>[6x]MPEQAVTLEALYAAIEQVLRERLPEAQLIGFWPGVPENTPAVSLEIAELLPERDPGTGESALLCRLQARIMVPPGADRQAVSIACGIVRTLREQTWNLSLQPARFVRSAVDGSREELKSLRVWLVEWTQSLRLGDPEWAWEDQPPGSLMLGFDPQTGPGHEPDYFAPEALA;>[18x]MSFFHGVTVTNVDIGARTIALPASSVIGLCDVFTPGAQASAKPNVPVLLTSKKDAAAAFGIGSSIYLACEAIYNRAQAVIVAVGVETAETPEA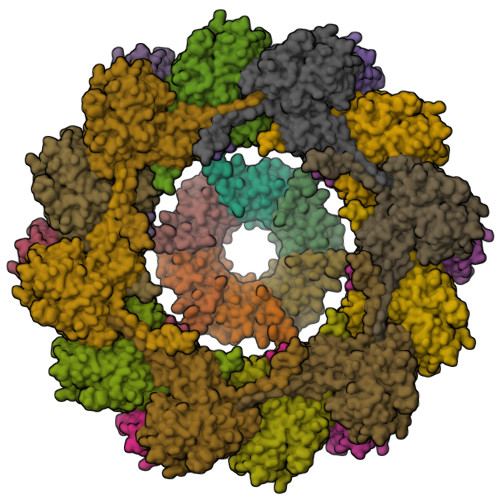QASAVIGGISAAGERTGLQALLDGKSRFNAQPRLLVAPGHSAQQAVATAMDGLAEKLRAIAILDGPNSTDEAAVAYAKNFGSKRLFMVDPGVQVWDSATNAARNAPASAYAAGLFAWTDAEYGFWSSPSNKEIKGVTGTSRPVEFLDGDETCRANLLNNANIATIIRDDGYRLWGNRTLSSDSKWAFVTRVRTMDLVMDAILAGHKWAVDRGITKTYVKDVTEGLRAFMRDLKNQGAVINFEVYADPDLNSASQLAQGKVYWNIRFTDVPPAENPNFRVEVTDQWLTEVLDVA>GSHMATNDELKNQLANKQNGGQVASAQSLDLKGLLEAPTMRKKFEKVLDKKAPQFLTSLLNLYNGDDYLQKTDPMTVVTSAMVAATLDLPIDKNLGYAWIVPYKGRAQFQLGYKGYIQLALR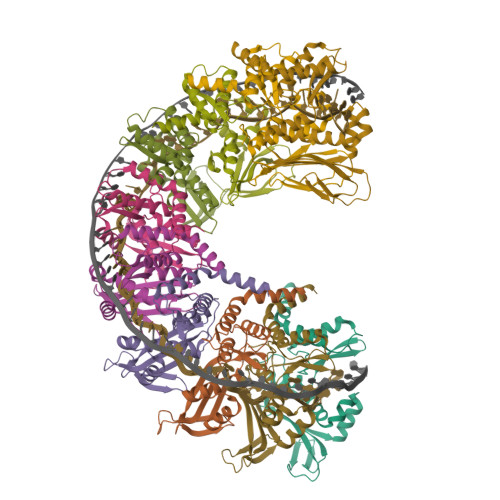TGQYKSINVIEVREGELLKWNRLTEEIELDLDNNTSEKVVGYCGYFQLINGFEKTVYWTRKEIEAHKQKFSKSDFGWKKDYDAMAKKTVLRNMLSKWGILSIDMQTAVTEDEAEPRERKDVTDDESIPDIIDAPVTPSDTLEAGSVVQGSMI[10x]> 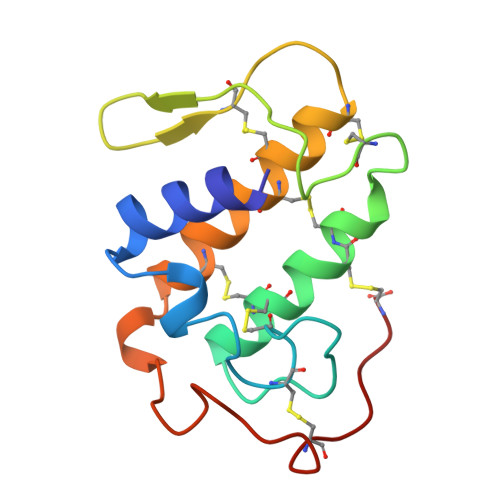SMYQLWKMILQETGKNAVPSYGLYGCNCGVGSRGKPKDATDRCCFVHKCCYKKLTDCSPKTDSYSYSWKDKTIVCGDNNPCLQEMCECDKAVAICLRENLDTYNKNYKIYPKPLCKKADAC> FPVPPSVDWREKGALVPIKNQGRCGSCWAFSAVASVEALNKIKGGELISLSEQMMVDCVNASYGCKGGRQTDAFKY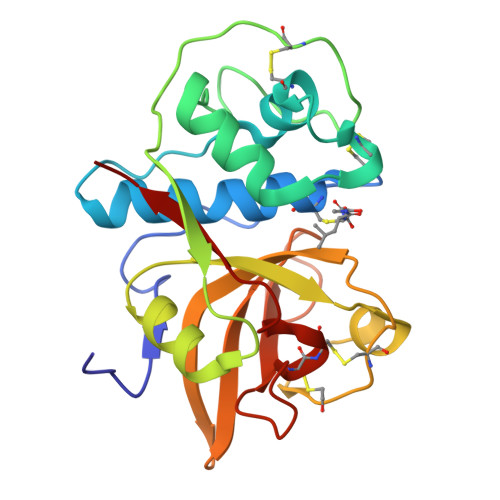IKVHGIASSKDYPYVGVQGPCQPKEIVLKISGYRGIVRNNEKYLQIIASQQVVSISIKVGKDFQHYKSGIFNGTCGDKINHGVNVVGYGSENGIPYWIVRNSWGKGWGEQGYIRMRRNTSNPAGCCGVAITPTFPVID> EDPEVLFKNKGCV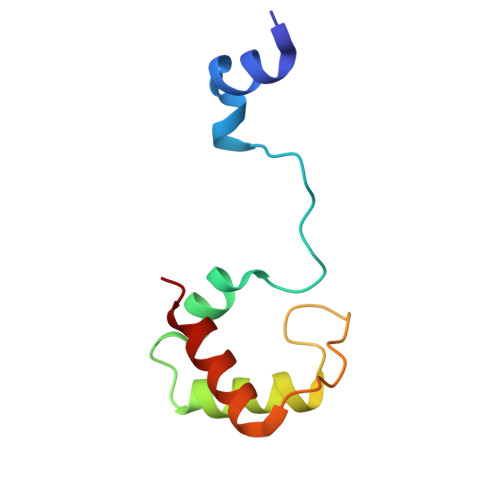ACHAIDTKKVGPAYADVAKKYAGRKDAVDYLAGKIKKGGSGVWGSVPMPPQNVTDAEAKQLAQWILSIK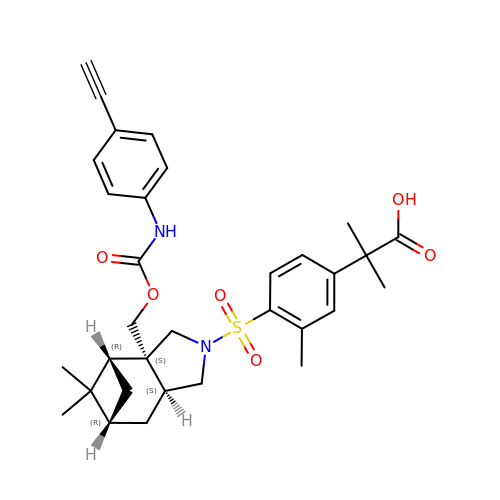2-[4-[[(1~{R},2~{S},6~{S},8~{R})-2-[(4-ethynylphenyl)carbamoyloxymethyl]-9,9-dimethyl-4-azatricyclo[6.1.1.0^{2,6}]decan-4-yl]sulfonyl]-3-methyl-phenyl]-2-methyl-propanoic acid | C32 H38 N2 O6 S | ZYKXPAJTMSTJLX-GXMIFEBGSA-N> MAMHPRKDWYELTRATNWTPSYVTEEQLFPERMSGHMGIPLEKWESYDEPYKTSYPEYVSIQREKDAGAYSVKAALERAKIYENSDPGWISTLKSHYGAIAVGEYAAVTGEGRMARFSKAPGNRNMATFGMMDELRHGQLQLFFPHEYCKKDRQFDWAWRAYHSNEWAAIAAKHFFDDIITGRDAISVAIMLTFSFETGFANMQFLGLAADAAEAGDYTFANLISSIQTDESRHAQQGGPALQLLIENGKREEAQKKVDMAIWRAWRLFAVLTGPVMDYYTPLEDRSQSFKEFMYEWIIGQFERSLIDLGLDKPWYWDLFLKDIDELHHSYHMGVWYW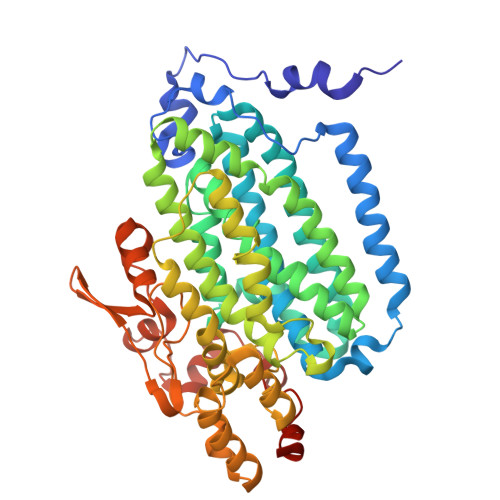RTTAWWNPAAGVTPEERDWLEEKYPGWNKRWGRCWDVITENVLNDRMDLVSPETLPSVCNMSQIPLVGVPGDDWNIEVFSLEHNGRLYHFGSEVDRWVFQQDPVQYQNHMNIVDRFLAGQIQPMTLEGALKYMGFQSIEEMGKDAHDFAWADKCKPAMKKSA> MTIKVGINGFGRIGRIVFRAAQKRSDIEIVAINDLLDADYMAYMLKYDSTHGRFDGTVEVKDGHLIVNGKKIRVTAERDPANLKWDEVGVDVVAEATGLFLTDETARKHITAGAKKVVMTGPSKDNTPMFVKGANFDKYAGQDIVSNASCTTNCLAPLAKVINDNFGIIEGLMTTVHATTATQKTVDGPSHKDWRGGRGASQNIIPSSTGAAKAVGKVLPELNGKLTGMAFRVPTPNVSVVDLTVRL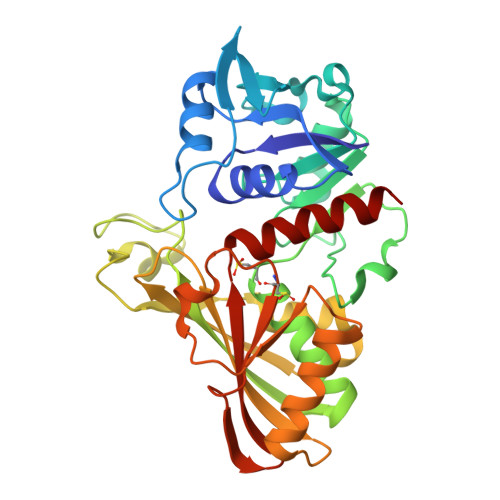EKAATYEQIKAAVKAAAEGEMKGVLGYTEDDVVSTDFNGEVCTSVFDAKAGIALNDNFVKLVSWYDNETGYSNKVLDLIAHISK> HHHHHHMFIEEFEIESITST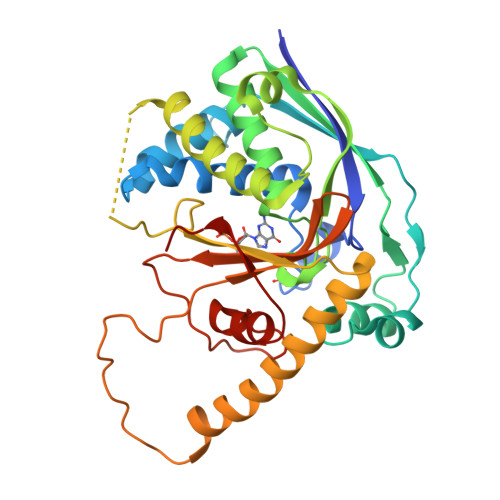HLLEVLTREYPEVRSPSIKGAMRWWFRALAGSYFGDDAQKLKEIENQVFGSTKERSRVKISVTPLSSPKRLNLKEFKDKNVGYIWFSINLLGKRGTITHYYPPGSRFRVVLESPSERVIKLATLSLWALVSLGSVGFRSRRGTGSMKIVRASSEVLEDLGLTTEFNSIDEFKDSLKRVLDVTGEILGVKNSETNKSLPSYATLKFSDVEVFGPGKNTWEVLAQFNNSYKEYLRRRIKKYQRIIFGLPRFKLRGVRKDLRRASPLWFGVVEIGGKPYGRIIKFFQSTFHPEVRSKHIVDWNVLSNFDWFISSRLPVTKVWGGWSG>FVSSHRYVETMLVADQSMAEFHGSGLKHYLLTLFSVAARLYKHPSIRNSVSLVVVKILVIHDEQKGPEVTSNAALTLRNFCNWQKQHNPPSDRDAEHYDTAILFTRQDLCGSQTCDTLGMADV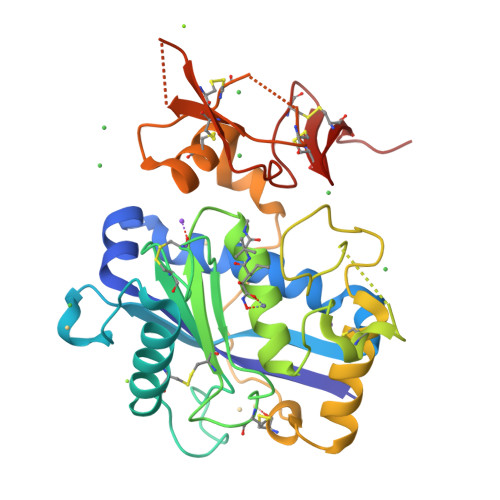GTVCDPSRSCSVIEDDGLQAAFTTAHELGHVFNMPHDDAKQCASLNGVNQDSHMMASMLSNLDHSQPWSPCSAYMITSFLDNGHGECLMDKPQNPIQLPGDLPGTSYDANRQCQFTFGEDSKHCPDAASTCSTLWCTGTSGGVLVCQTKHFPWADGTSCGEGKWCINGKCVNKLVPR[2x]> GSFMKTIGIFYATLTGTTVGIVDEIEFFLKKDDFKTFNVKN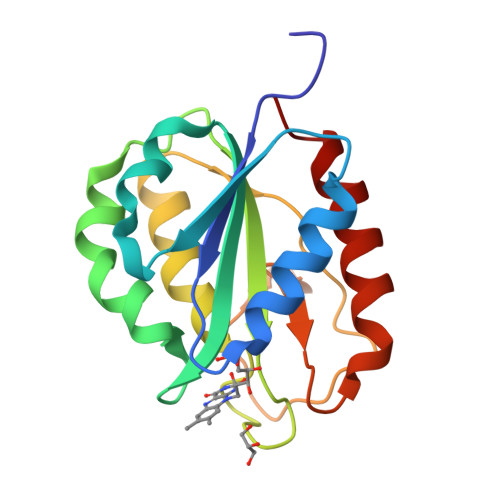GVKEIENFENLILVTPTYQVGEAHAAWMNNLKKLEEIDFTGKVVGLVGLGNQFAFGESFCGGIRYLYDIVVKKGGKVVGFTSTDGYHYEETSIIENGKFIGLALDEENQPNLTPKRIGDWITEIKKEFK>[12x]MRFWP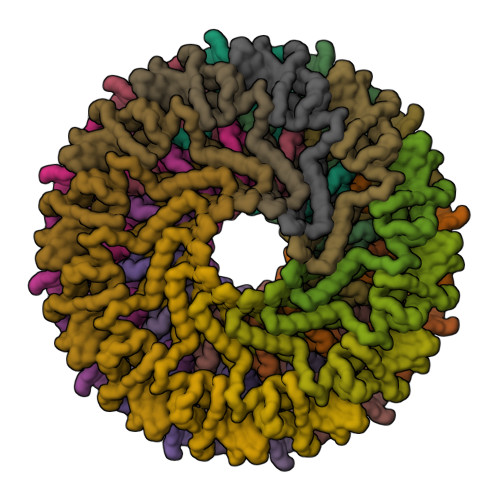FSKTTNAATRAEPMVTRPDTAPRVRSYRAAKSDRIAGGFGVFPTTPRDELRREIRGLVGHSRHAAQNFDYARAYEMLTRRHVIGFNGIRLQMDVRDPGGKKDVAAGAQIESAWARWGKMKNSPTPCGRLSWWGVECQVATGIAREGGSFVRIHQGTNRGRFGFQVEPIPFDLLDLDLTGPTPGGGFVGIAREGGSFVRIHQGTNRGRFGFQVEPIPFDLLDLDLTGPTPGGGFVESGVEFDATDRVVAYHMWSAAMSEGHRPGARRRLRIPAAQMLYVLVPEEIGQALGVPRSATALRLMNLSEKFQESALTAANYGASNMVFFERAADNGVVTGPEDDAQIPIDQIEAGTLTELPPGVKAVSHNPAYPDAAVGPFLRQMGTSQAAGLGVSYETLTADLSGANFSSLRAGKGEEREEWRMLQRAVFEGLHDRVFSRWLPLAMLSGEVRLPLAKLDKFDAATWRPRGWPSVNPKDDATAHEKDLKNGVRTRTEICAERGRDFADVVAEAAAERQMMRDAGLDPDAPLRTSPPETPPDPGEEIEGKDT;>MTVSIHPPATLVAGDSWAWEAGAVFEDHPDPWAASYVLRPEAGGDPVTVSGGLEVLAPVFRLPASVTADLPPGEWTWFAVAVDATTDARAVLAQGRVTVIPDPLAGTEDRRTPARRILAAIEATLEGRATKDADTYSIEGRSITRTPLPDLLRLRAVYAEQVARETGRSPYRQRRVSF[12x]2-acetamido-2-deoxy-6-O-phosphono-alpha-D-glucopyranose | C8 H16 N O9 P | 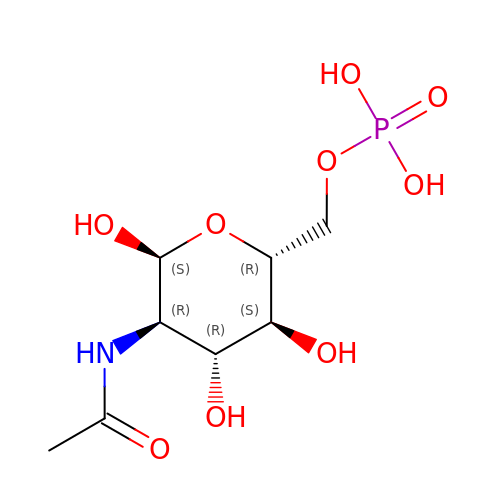BRGMHAYQAZFZDJ-PVFLNQBWSA-N> GAMGPQEYTLIKLKIHLIPEFLGSIVKGREVFVVCATLRPETMYGQTNCWILPDGEYDLVLAFDQVIPYDAKTSDGVLCKIFDKYEDTMKECNTVYICSERSAYNMAYQGIVPLIHGREQGVSDKLLPRIVSLGKVYGEQLIGTPLSAPMTPYSLIFILPMFSISMEKGTGIVTSVPSDSPDDYAALRDIKTKPLLREKYSIKDEWILDPLEIIEVPGFGFMTAELLCNQYKIQSQNDSAKLKQAKEEIYKKEFYEGILIRGKYSGMKICDAKELIRESLI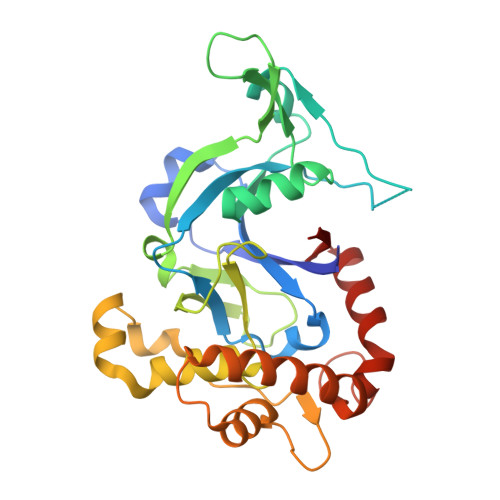KDGYALIYLE> 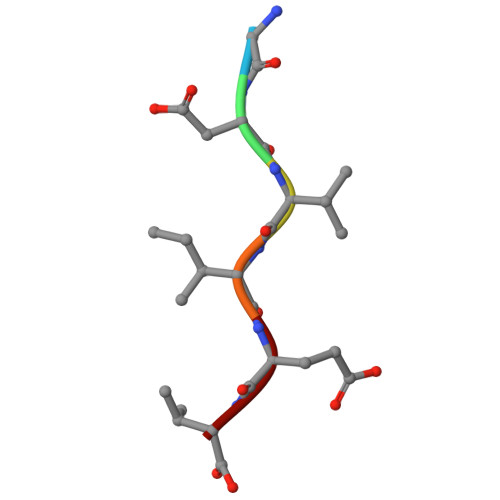GDVIEV> MSVKASGGSSLARPQLYQTVPVSAISQAEQQDRFLEGSELNELTAYFQSGALRLEIAETLTQNADLIVSRAANRIFTGGSPLSYLEKPVERQPALVGASSDSRNGSVTYAESNGSGGLFGGLRSVFSSTGPIPPGFRPINIARYGPSNMQKSLRDMSWFLRYTTYAIVAGDPNIIVVNTRGLKEVIENACSIDATIVAIQEMRAASADYFRNNAQAKEIVLQYFDILLSEFKAPTPANKVRQGPSNDIQGLELPQSYFNAAAKRQKYAMKPGLSALEKNA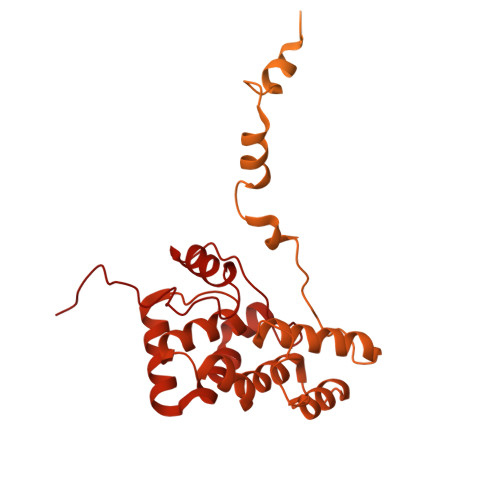VIKAAYRQIFERDITKAYSQSISYLESQVRNGDISMKEFVRRLAKSPLYRKQFFEPFINSRALELAFRHILGRGPSSREEVQKYFSIVSSGGLPALVDALVDSQEYADYFGEETVPYLRGLGVEAQECRNWGMQQDLFSYSAPFRKVPQFITTFAQYDRPLPDQHVYGSGNDPLEIQFGAIFPKETRNPSKRPAPFNKDTKRILIHRGPAVNNQVGNPSAVGEFPGSLGAKVFRLNGGLPGAKVGKNTGTSVKFGESSTQALIRAAYRQVFGRDLYEGQRLSVAEIQLENGDISVREFIKRLAKSELFLKLYWAPHYVCKAIEYMHRRLLGRPTYGRQEMNQYFDIASKQGFYAVVEAMIDSKEYSDAFGEDTVPYERYLTPGGLQMRSARVGSLREDIGQRVDKEVTPRFVELGQVSAIRTEPEIAYRSNQGVTRQRQQTKVFKLVSTYDKVAVKNAIRAAYRQVFERDLEPYIINSEFTALESKLSNNEINVKEFIEGLGTSELYMKEFYAPYPNTKVIEMGTKHFLGRAPLNQKEIQQYNQILASQGLKAFIGAMVNGMEYLQTFGEDTVPYRRFPTLPAANFPNTERLYNKLTKQDKELVVPSFTPVVKVGG>[18x]GAMGNQKTKASKLETAAKNLENQNKQEYIKINEIDAQGINFLATFKADEKDNLSQYEEMQIKRTIYSSLNYEKQKIN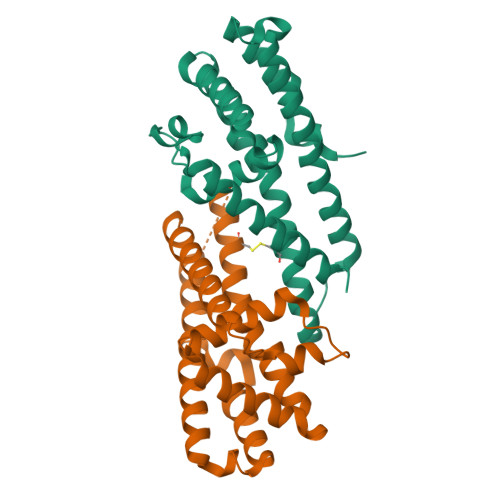TLKEILETLYNKLQHRYTSKEFIYQIVASIQYDIDRVLCLIKEAIIKDNLHTQNQKESELLMNLDSSLKTRQNFAKKLNETIDDYNKDSKNIQTNVDALATYMKENYKTLDSFKPIN>GMVTTRKPLRAAIIGLGRLGERHARHLVNKIQGVKLVAACALDSNQLEWAKNELGVETTYTNYKDMIDTENIDAIFIVAPTPFHPEMTIYAMNAGLNVF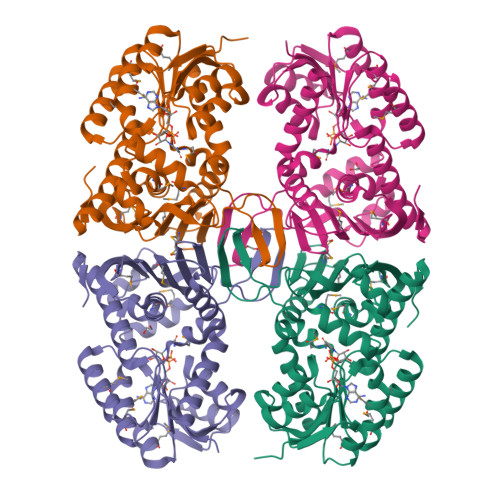CEKPLGLDFNEVDEMAKVIKSHPNQIFQSGFMRRYDDSYRYAKKIVDNGDIGKIIYMRGYGIDPISGMESFTKFATEADSGGIFVDMNIHDIDLIRWFTGQDPVQAYGLTSNIAAPQLADIGEFETGVAQLKMSDGVIATLIGGRHAAHGNQVELEVMGSNGWVRIGEHPDLNRVTVFNDQGVVRPSLQSFGERFDTAFTDEVQDFVNNVIVGKQPEVTVDDGIKALKIAKACQQSANIGKLVDIQL[4x]>[16x]MTTVSCPANVITTTESDRIAGLFNIPAGIIPTGNVLSTIEVCAHRCIFDFFKQIRSDDNSLYSAQFDILLGTYCNTLNFVRFLELGLSVACICTKFPELAYVRDGVIQFEVQQPMIARDGPHPVDQPVHNYMVKRIHKRSLSAAFAIASEALSLLSNTYVDGTEIDSSLRIRAIQQMARNLRTVLDSFERGTADQLLGVLLEKAPPLSLLSPINKFQPEGHLNRVARAALLSDLKRRVCADMFFMTRHAREPRLISAYLSDMVSCTQPSVMVSRITHTNTRGRQVDGVLVTTATLKRQLLQGILQIDDTAADVPVTYGEMVLQGTNLVTALVMGKAVRGMDDVARHLLDITDPNTLNIPSIPPQSNSDSTTAGLPVNARVPADLVIVGDKLVFLEALERRVYQATRVAYPLIGNIDITFIMPMGVFQANSMDRYTRHAGDFSTVSEQDPRQFPPQGIFFYNKDGILTQLTLRDAMGTICHSSLLDVEATLVALRQQHLDRQCYFGVYVAEGTEDTLDVQMGRFMETWADMMPHHPHWVNEHLTILQFIAPSNPRLRFELNPAFDFFVAPGDVDLPGPQRPPEAMPTVNATLRIINGNIPVPLCPISFRDCRGTQLGLGRHTMTPATIKAVKDTFEDRAYPTIFYMLEAVIHGNERNFCALLRLLTQCIRGYWEQSHRVAFVNNFHMLMYITTYLGNGELPEVCINIYRDLLQHVRALRQTITDFTIQGEGHNGETSEALNNILTDDTFIAPILWDCDALIYRDEAARDRLPAIRVSGRNGYQALHFVDMAGHNFQRRDNVLIHGRPVRGDTGQGIPITPHHDREWGILSKIYYYIVIPAFSRGSCCTMGVRYDRLYPALQAVIVPEIPADEEAPTTPEDPRHPLHAHQLVPNSLNVYFHNAHLTVDGDALLTLQELMGDMAERTTAILVSSAPDAGAATATTRNMRIYDGALYHGLIMMAYQAYDETIATGTFFYPVPVNPLFACPEHLASLRGMTNARRVLAKMVPPIPPFLGANHHATIRQPVAYHVTHSKSDFNTLTYSLLGGYFKFTPISLTHQLRTGFHPGIAFTVVRQDRFATEQLLYAERASESYFVGQIQVHHHDAIGGVNFTLTQPRAHVDLGVGYTAVCATAALRCPLTDMGNTAQNLFFSRGGVPMLHDNVTESLRRITASGGRLNPTEPLPIFGGLRPATSAGIARGQASVCEFVAMPVSTDLQYFRTACNPRGRASGMLYMGDRDADIEAIMFDHTQSDVAYTDRATLNPWASQKHSYGDRLYNGTYNLTGASPIYSPCFKFFTPAEVNTNCNTLDRLLMEAKAVASQSSTDTEYQFKRPPGSTEMTQDPCGLFQEAYPPLCSSDAAMLRTAHAGETGADEVHLAQYLIRDASPLRGCLPLPR;>[15x]MTQPASSRVVFDPSNPTTFSVEAIAAYTPVALIRLLNASGPLQPGHRVDIADARSIYTVGAAASAARARANHNANTIRRTAMFAETDPMTWLRPTVGLKRTFNPRIIRPQPPNPSMSLGISGPTILPQKTQSADQSALQQPAALAFSGSSPQHPPPQTTSASVGQQQHVVSGSSGQQPQQGAQSSTVQPTTGSPPAAQGVPQSTPPPTQNTPQGGKGQTLSHTGQSGNASRSRRV;>MGSQPTNSHFTLNEQTLCGTNISLLGNNRFIQIGNGLHMTYAPGFFGNWSRDLTIGPRFGGLNKQPIHVPPKRTETASIQVTPRSIVINRMNNIQINPTSIGNPQVTIRLPLNNFKSTTQLIQQVSLTDFFRPDIEHAGSIVLILRHPSDMIGEANTLTQAGRDPDVLLEGLRNLFNACTAPWTVGEGGGLRAYVTSLSFIAACRAEEYTDKQAADANRTAIVSAYGCSRMETRLIRFSECLRAMVQCHVFPHRFISFFGSLLEYTIQDNLCNITAVAKGPQEAARTDKTSTRRVTANIPACVFWDVDKDLHLSADGLKHVFLVFVYTQRRQREGVRLHLALSQLNEQCFGRGIGFLLGRIRAENAAWGTEGVANTHQPYNTRALPLVQLSNDPTSPRC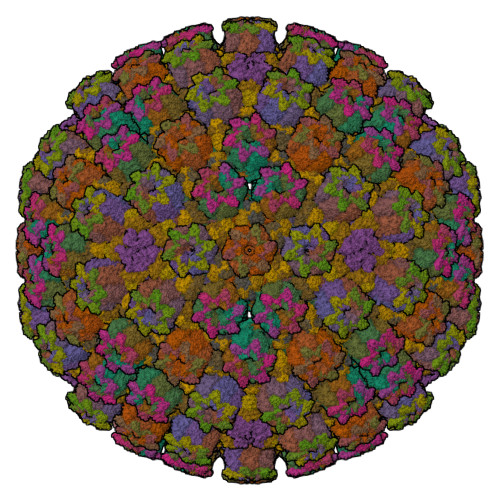SIGEITGVNWNLARQRLYQWTGDFRGLPTQLSCMYAAYTLIGTIPSESVRYTRRMERFGGYNVPTIWLEGVVWGGTNTWNECYY[5x];>MAMPFEIEVLLPGELSPAETSALQKCEGKIITFSTLRHRASLVDIALSSYYINGAPPDTLSLLEAYRMRFAAVITRVIPGKLLAHAIGVGTPTPGLFIQNTSPVDLCNGDYICLLPPVFGSADSIRLDSVGLEIVFPLTIPQTLMREIIAKVVARAVERTAAGAQILPHEVLRGADVICYNGRRYELETNLQHRDGSDAAIRTLVLNLMFSINEGCLLLLALIPTLLVQGAHDGYVNLLIQTANCVRETGQLINIPPMPRIQDGHRRFPIYETISSWISTSSRLGDTLGTRAILRVCVFDGPSTVHPGDRTAVIQV[10x]> GSVKPTQQARPTVIRWSEGGKEVFISGSFNNWSTKIPLIKSHNDFVAILDLPEGEHQYKFFVDGQWVHDPSEPVVTSQLGTINNLIH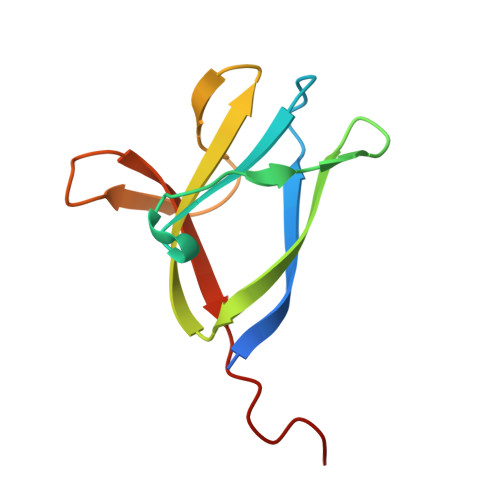VKKSDFEVF>MDTALERQIASASRSVEEARRLAYHDPIRVGALVEQISVLADLRQKEGDFRKAESLYREALFRAQELRKQDPDLLTGIYSLLAHLYDRWGRMDKAAEFYELALKISAENGLEESDKVATIKNNLAMIFKQLRKFERAEGYYCEALETFQRLDGEQSARVASVYNNLGVLYYSHMDVDRAQVMHERALAIRQNLHEGQMDPADLSQTFINLGAVY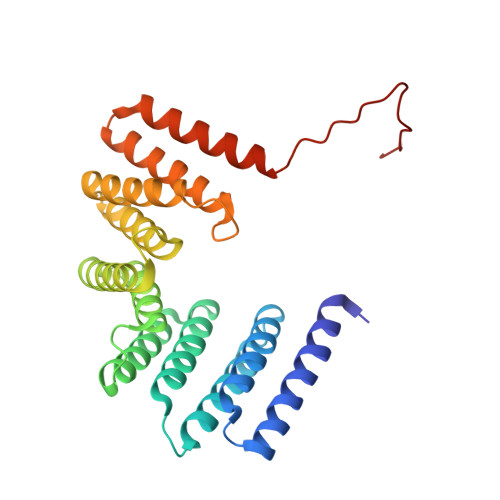KAAGDFQKAEACVDRAKRIRAAMNGYHPNPRRSASLLIDKSL[2x]(2S)-2-methyl-3-sulfanyl-propan-1-ol | C4 H10 O S | 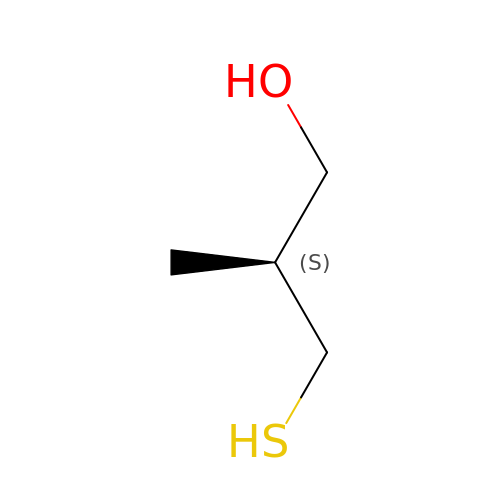FCIVYWQHILCTLI-BYPYZUCNSA-N> GSFTMGRLYSGNLAAFKAATNKLFQLDLAVIYDDWYDAYTRKDCIRLRIEDRSGNLIDTSTFYHHDED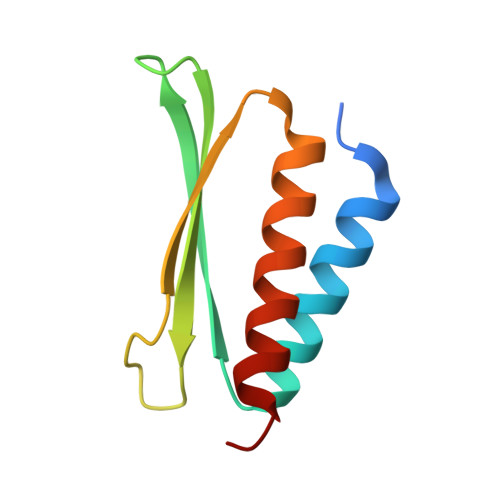VLFNMCTDWLNHMYDQLKDWK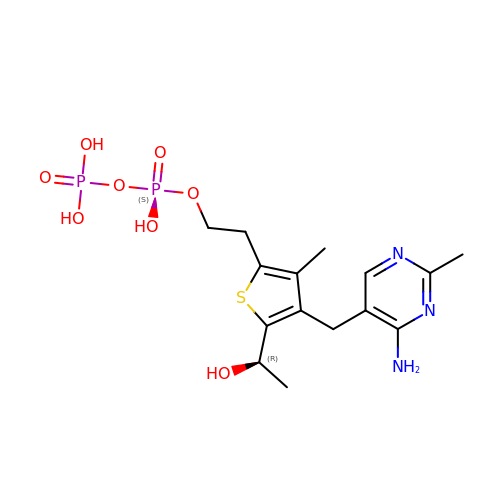2-{4-[(4-AMINO-2-METHYLPYRIMIDIN-5-YL)METHYL]-5-[(1R)-1-HYDROXYETHYL]-3-METHYL-2-THIENYL}ETHYL TRIHYDROGEN DIPHOSPHATE | C15 H23 N3 O8 P2 S | ORVRYSKZCUVOLA-SECBINFHSA-N>MAKTQAEINKRLDAYAKGTVDSPYRVKKATSYDPSFGVMEAGAIDADGYYHAQCQDLITDYVLWLTDNKVRTWGNAKDQIKQSYGTGFKIHENKPSTVPKKGWIAVFTSGSYEQWGHIGIVYDGGNTSTFTILEQNWNGYANKKPTKRVDNYYGLTHFIEIPVKA[4x]

LysK, an endolysin from staphylococcal phage K, contains an N-terminal cysteine-histidine dependent amido-hydrolase/peptidase domain (CHAPK), a central amidase domain and a C-terminal SH3b cell wall-binding domain. CHAPK cleaves bacterial peptidoglycan between the tetra-peptide stem and the penta-glycine bridge. The structure has the papain-type fold with a long loop between the two amino-terminal alpha-helices. The structure suggests the location of the active site near a hydrophobic groove, with Cys54, His117 and Glu134 forming the catalytic triad.

For the derivative structure, a calcium ion and a 2-[4-(2-hydroxyethyl)piperazin-1-yl] ethanesulfonic acid (HEPES) molecule have been modelled associated with each of the protein chains, while Cys54 is modelled as methylmercury-cysteine. In this case, ordered solvent molecules modelled in the unit cell include two glycerol molecules, ten additional putative methylmercury ions, two putative chloride ions and 770 waters. In the derivative protein structure, the calcium is present at the same occupancy and with the same coordinating ligands. In contrast to the tightly bound calcium ion, the zinc ions appear to be bound more loosely and the derivative structure shows they could be replaced by methylmercury ions upon soaking of the crystals with methylmercury chloride. A zinc ion was also found and is likely more loosely bound, as it is less buried, has less protein ligands and could be exchanged for a methylmercury ion upon derivatization. In both structures, a buffer molecule occupies the groove that likely accommodates the peptidoglycan substrate: a Bis-Tris molecule (2-[Bis(2-hydroxyethyl)amino]-2-(hydroxymethyl)-1,3-propanediol) in between the two monomers of the asymmetric unit of CHAPGH15 and a MES and HEPES molecule in the case of the native and derivative structures of CHAPK, respectively.> MTDQIDKDAQNTHELTTRVARALIARGWRLTTAESCTGGNLAAALCAQADTAAFYDTGVVTFSDEAKRNVLQVRAETLAVHSA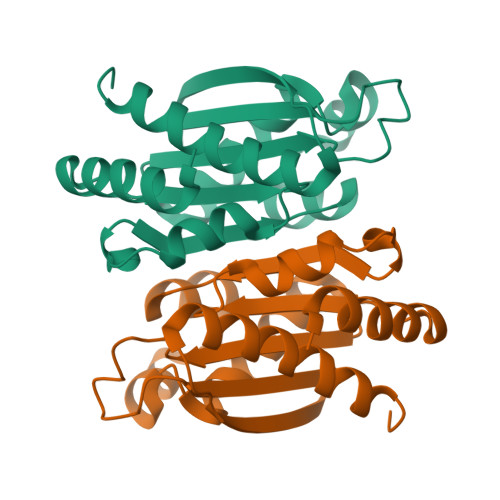VSEACVQEMSTGILTLAGADIAIAISGYAGPEGGEDGTPAGTVWFAWNFRGQIETQRMRFTGDCEAVVAQAVRFAMAALGEKLAHWQ(3-phenyl-1,2-oxazol-5-yl)methylazanium | C10 H11 N2 O | 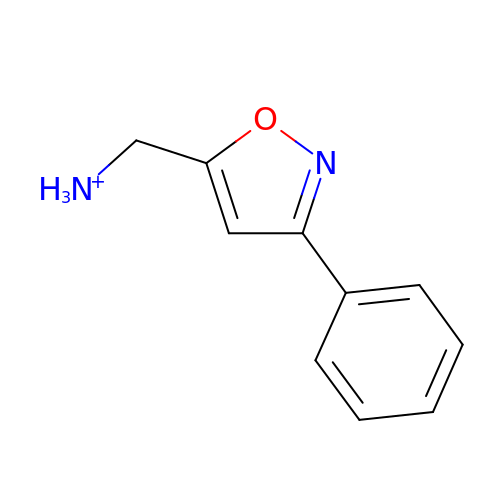AQZLTCXQTOKUAA-UHFFFAOYSA-O> SKYSQDVLQLLYKNKPNYISGQSIAESLNISRTAVKKVIDQLKLEGCKIDSVNHKGHLLQQLPDIWYQGIIDQYTKSSALFDFSEVYDSIDSTQLAAKKSLVGNQSSFFILSDEQTKGRGRFNRHWSSSKGQGLWMSVVLRPNVAF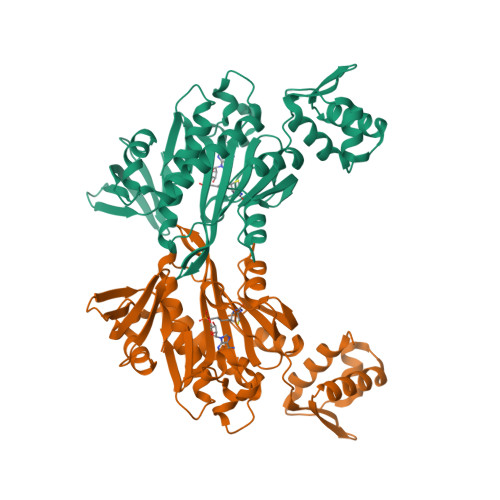SMISKFNLFIALGIRDAIQHFSQDEVKVKWPNDIYIDNGKVCGFLTEMVANNDGIEAIICGIGINLTQQLENFDESIRHRATSIQLHDKNKLDRYQFLERLLQEIEKRYNQFLTLPFSEIREEYIAASNIWNRTLLFTENDKQFKGQAIDLDYDGYLIVRDEAGESHRLISADIDFHHHHHH>[2x]MPKYVEGVELTQEGMHAIFARMGYGDITSGSIYNGVPTIDTGALNRQGFMPVLTGVGPHR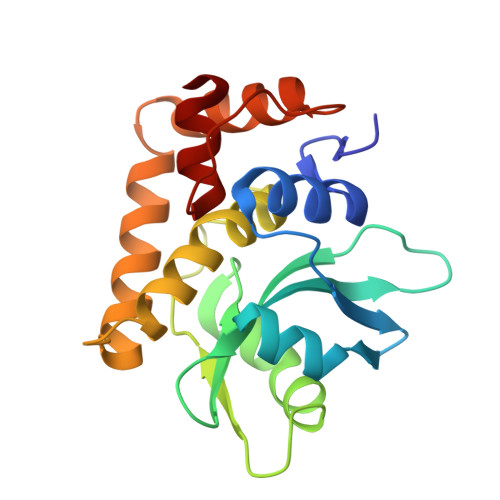DSGHWIMLIKGPGNQYYLFDPLGKTSGEGYQNILAAQLPMGSTLSVIPNGSGLNMGLCGYWVASAGLRAHQALNQHNPPTLLNVGQTITNEMRNELDHDGYRKITGWLRAVADEFPEGDPQLDGKALRENTEK> MFENITAAPADPILGLADLFRADERPGKINLGIGVYKDETGK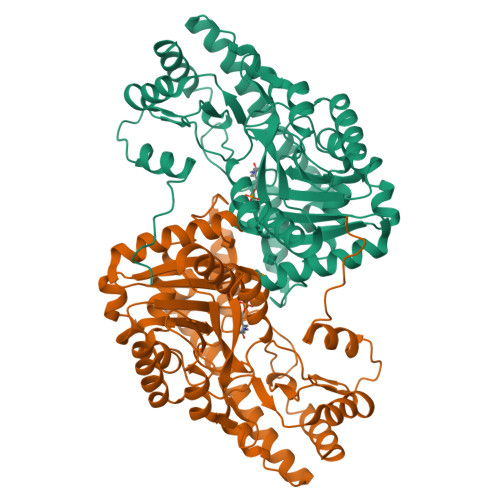TPVLTSVKKAEQYLLENETTKNYLGIDGIPEFGRCTQELLFGKGSALINDKRARTAQTPGGTGALRVAADFLAKNTSVKRVWVSNPSWPNHKSVFNSAGLEVREYAYYDAENHTLDFDALINSLNEAQAGDVVLFHGCCHAPTGIDPTLEQWQTLAQLSVEKGWLPLFDFAYQGFARGLEEDAEGLRAFAAMHKELIVASSYSKNFGLYNERVGACTLVAADSETVDRAFSQMKAAILANYSNPPAHGASVVATILSNDALRAIWEQELTDMRQRIQRMRQLFVNTLQEKGANRDFSFIIKQNGMFSFSGLTKEQVLRLREEFGVYAVASGLVNVAGMTPDNMAPLCEAIVAVL> MHHHHHHENLYFQGTVVTTESGLKYEDLTEGSGAEARAGQTVSVHYTGWLTDGQKFDSS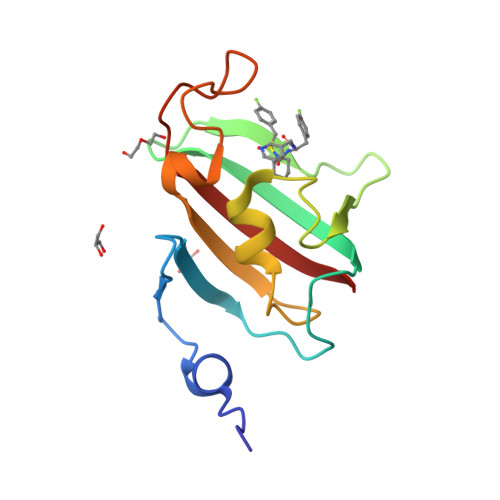KDRNDPFAFVLGGGMVIKGWDEGVQGMKVGGVRRLTIPPQLGYGARGAGGVIPPNATLVFEVELLDV>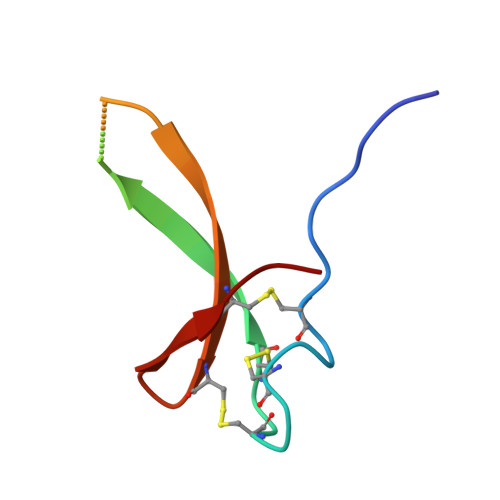 AGSRLPDCSHACGSCSPCRLVMVSFVCASVEEAETCPMAYKCMCNNKSYPVP> DREEAAFLAASILIQHAHEQGKDDRELEKILEIAIRILEKNGVDREEAAFLAASILIQHAHEQGKDDRELEKILEIAIRILEKNGVDREEAAFLAASILIQHAHEQGKDDRELEKILEIAIR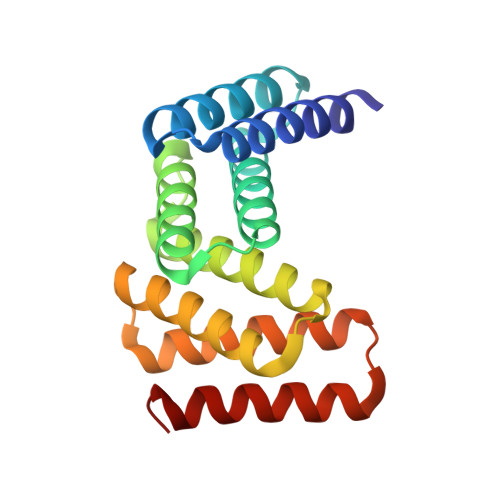ILEKNGVDREEAAFLAASILIQHAHEQGKDDRELEKILEIAIRILEKNGV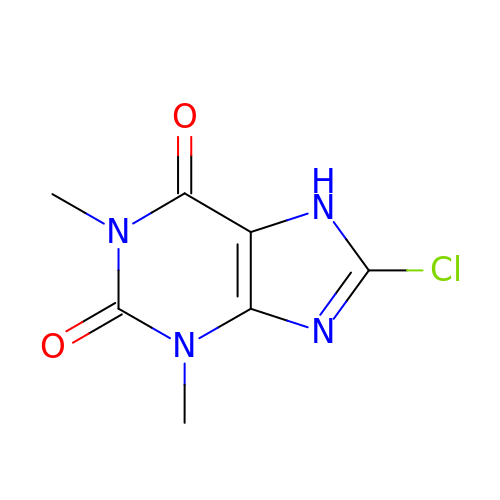8-CHLORO-1,3-DIMETHYL-3,7-DIHYDRO-1H-PURINE-2,6-DIONE | C7 H7 Cl N4 O2 | RYIGNEOBDRVTHA-UHFFFAOYSA-N PHOSPHORIC ACID 2-AMINO-3-(4-HYDROXY-PHENYL)-PROPYL 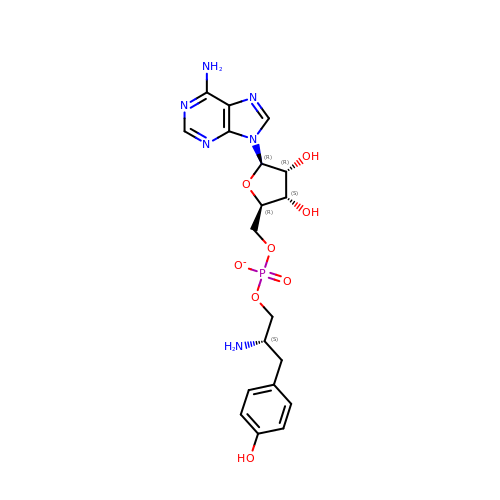ESTER ADENOSIN-5'YL ESTER | C19 H24 N6 O8 P | JJLCVHBFTXDJMM-KFAHYOAQSA-M> SGPQIKELTDEEAERLQLEIDQKKDAENHEA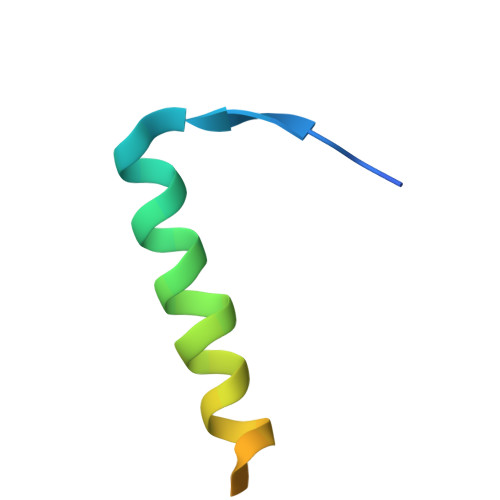QLKNGSLDSPG ethyl 2-methyl-1,3-thiazole-4-carboxylate | C7 H9 N O2 S | 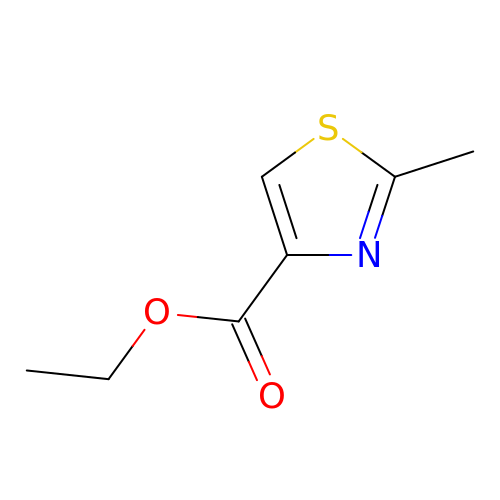QWWPUBQHZFHZSF-UHFFFAOYSA-N>MISILRRGLLVLLAAFPLLALAVQTPHEVVQSTTNELLGDLKANKEQYKSNPNAFYDSLNRILGPVVDADGISRSIMTVKYSRKATPEQMQRFQENFKRSLMQFYGNALLEYNNQGITVDPAKADDGKRASVGMKVTGNNGAVYPVQYTLENIGGEWKVRNVIVNGINIGKLFRDQFADAMQRNGNDLDKTIDGW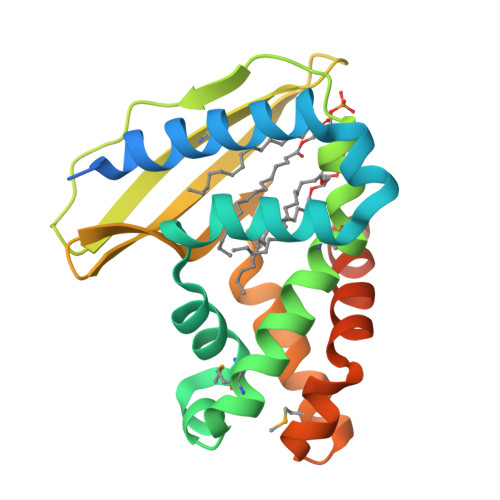AGEVAKAKQAADNSPEKSVKLEHHHHHH[2x]> SAEKLFTPLKVGAVTAPNRVFMAPLTRLRSIEPGDIPTPLMGEYYRQRASAGLIISEATQISAQAKGYAGAPGLHSPEQIAAWKKITAGVHAEDGRIAVQLWHTGRISHSSIQPGGQAPVSASALNANTRTSLRDENGNAIRVDTTTPRALELDEIPGIVNDFRQAVANAREAGFDLVELHSAHGFLLHQFLSPSSNQRTDQYGGSVENRARLVLEVVDAVCNEWSADRIGIRVSPIGTFQNVDNGPNEEADALYLIEELAKRGIAY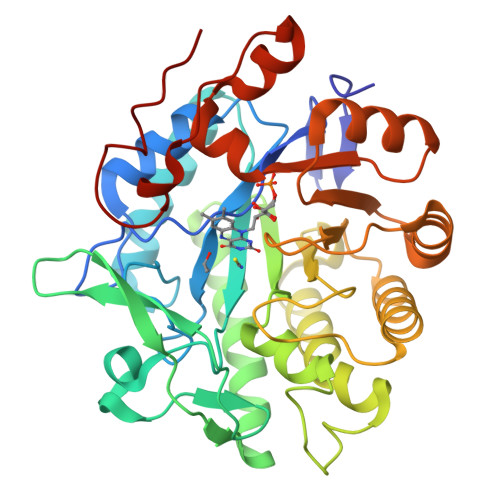LHMSETDLAGGKPYSEAFRQKVRERFHGVIIGAGAYTAEKAEDLIGKGLIDAVAFGRDYIANPDLVARLQKKAELNPQRPESFYGGGAEGYTDYPSL Here we identify and characterise a sub-family of multi-centre photoreceptors, termed photocobilins, that use B12 and biliverdin (BV) to sense light across the visible spectrum. We have identified and characterised two types of photocobilins, one from Saccharothrix syringae (SasPcob) that represents a standalone photocobilin photoreceptor and a more complex protein that consists of a photocobilin diguanylate cyclase (DGC) fusion from Acidimicrobiaceae bacterium (AbDPcob) that is representative of a photocobilin domain fused to an enzyme domain. Crystal structures reveal close juxtaposition of the B12 and BV chromophores, an arrangement that facilitates optical coupling. Light-triggered conversion of the B12 affects quaternary structure, in turn leading to light-activation of associated enzyme domains.

The adenosine binding pocket is strikingly similar, with the ribose moiety stacking with the conserved Trp61 residue and forming a network of polar interactions linking across the dimer interface via the conserved Glu71-His72 motif. In SasPcob, the BV is bound with a ZZZ configuration, with Asp270 forming key interactions with the co-planar A, B and C pyrrole rings. The D ring is positioned out of the ABC plane by approximately 40° due to close interactions with Trp296. In SasPcob, the close interaction and relative position of the B12- and BV-binding domains brings the two chromophores in close proximity, with the edge of the BV C and D rings within van der Waal’s distance of the conserved Trp61 and the corrin ring B, respectively. Furthermore, a direct hydrogen bond is formed between one of the corrin ring B amide groups and the BV ring D. This likely explains the B12 allosteric effects on BV affinity observed in solution. A network of direct and water mediated polar interactions surround this central chromophore edge-to-edge contact. These include direct hydrogen bonds between the corrin ring and Trp296 from the globin domain, and a putative salt bridge formed between the propionic acid of ring C of BV and His137 of the opposite monomer. The juxtaposition of both chromophores likely underpins the optical coupling observed.

>[2x]DILAAGREELMAALAEGDEHAAVDLAMRLLDGGVPADVVLLELVADAQVEIGVLWQANRWSVAQEHAATAISERVIAAVGDRAAAAPTRGHVVVACLDGEWHALPARIVAEVLRGRGWRVTFLGASVPAAHLVPYLEEHGPDAVALSCTLPRGLPRADQVVAACRATGTPVLVGGLGFGPDGRWARVLGAGTWAPTARAAADLLDRPEWPRTALPAPPRPADPEYAALRARRAELVDAGLAALHEWFPPLRDYDARRLDATLDDLGDIVDHLAASVYVDDPELFGEFVTWTAEVLAARGVSPASVEVALEAIARVLDDHPRTRHHLDHGRRALAAHLEH> KDSTESKSWEPFSLSPIKDPQALHKELCSKNVIPVTSTLEDLLPATQAQHVFIKRGTFHSYNWTIKGRSLNMDRLRETCQSLVDRHSILRTSFVEHEGHPIQLVLANLDVKVREVQCWPGEDPMEVCKALWDGKDWPTLNVLGGSLPVRFTLVSCPGNEHVVLTIQISHSQWDGVSIPKLFSDFAAIYNQTPLPPTSDFAHYLYHRVSSAREDVQQDPTFQFWRHYLDGAKMAVPFAPRALTLCAEPAAAAQSGQTLWTFKGIVPPTLPSGITMATL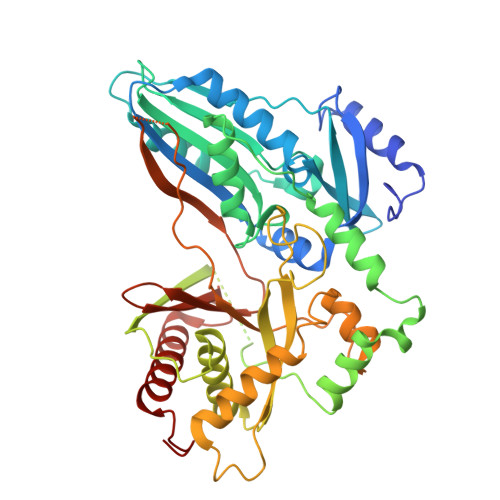VKAATALFLSYHLGSRDVVFGHTVNGRNLPMDNIESLLGCTLNFVPLRVTFPEDSTDWTVMDLLHHTQTQYTRALSHEHVELRDIFQHSTNWPAETPLSLIVQHQNIDLSFSLPLRGSSVSGDGEDDSSLDVQYSKFARFDPLDEVWIFTEPHADRLEVQVCANSRVLGQEQATELANNISAIITKFSTDPTARLLDITF>HMAVKKIAIFGATGQTGLTTLAQAVQAGYEVTVLVRDSSRLPSEGPRPAHVVVGDVLQAADVDKTVAGQDAVIVLLGTRNDLSPTTVMSEGARNIVAAMKAHGVDKVVACTSAFLLWDPTKVPPRLQAVTDDHIRMHKVLRESGLKYVAVMPPHIGDQPLTG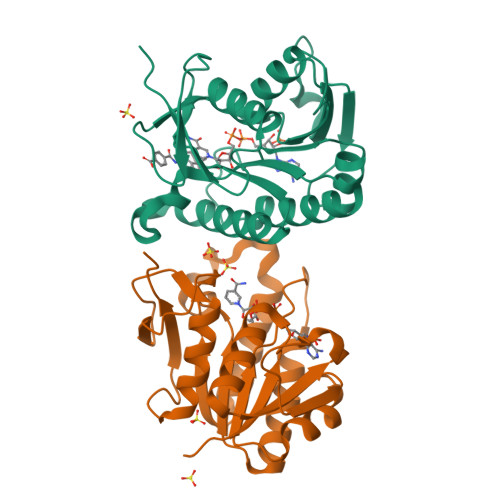AYTVTLDGRGPSRVISKHDLGHFMLRCLTTDEYDGHSTYPSHQYQ[2x]> DQVLKGAALVGHNVLVPSAQVAIDATGSAKGVVAATSAGFVNFEITDANGTFVKQLSVPASAAGEVSFAWDGTDAN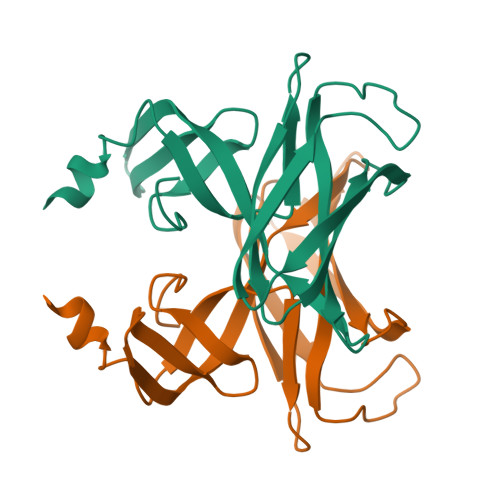GNRMAAGKYGITATQTDTAGAKSKLATYVDAPVDSVTIGSDGLYLNLTGLGTSPLANVLRVS6-amino-4-{2-[(cyclopentylmethyl)amino]ethyl}-2-(methylamino)-1,7-dihydro-8H-imidazo[4,5-g]quinazolin-8-one 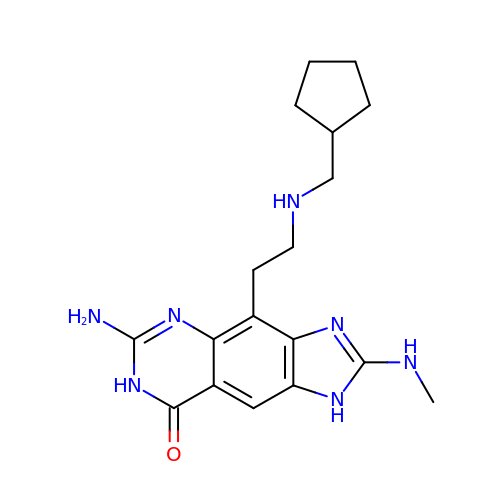| C18 H25 N7 O | OTRZFAIJJHPZSL-UHFFFAOYSA-N1-((2-HYDROXYETHOXY)METHYL)-5-(PHENYLSELANYL)PYRIMIDINE-2,4(1H,3H)-DIONE | C13 H14 N2 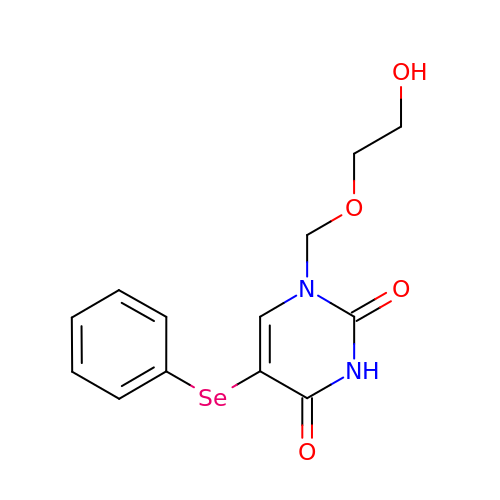O4 Se | KFSPSGWABMNFIY-UHFFFAOYSA-N>[2x]ETGDEDLPGAVPTESIQGSTFEEKIFLQWREPTQTYGVITLYEITYKAVSSFDPEIDLSNQSGRVSKLGNETHFLFFGLYPGTTYSFTIRASTAKGFGPPATNQFTTKISAPSMPAYELETPLNQTDNTVTVMLKPAHSRGAPVSVYQIVVEEERPRRTKKTTEILKCYPVPIHFQNASLLNSQYYFAAEFPADSLQAAQPFTIGDNKTYNGYWN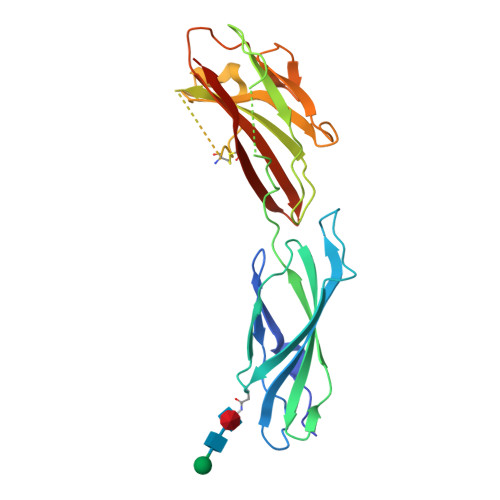TPLLPYKSYRIYFQAASRANGETKIDCVQVATKGGTKHHHHHH> TDKNQTTQNNSSSPLTQVNTTVSVQIGTKALLCCFSIPLTKAVLITWIIKLRGLPSCTIAYKVDTKTNETSCLGRNITWASTPDHSPELQISAVTLQHEGTYTCETVTPE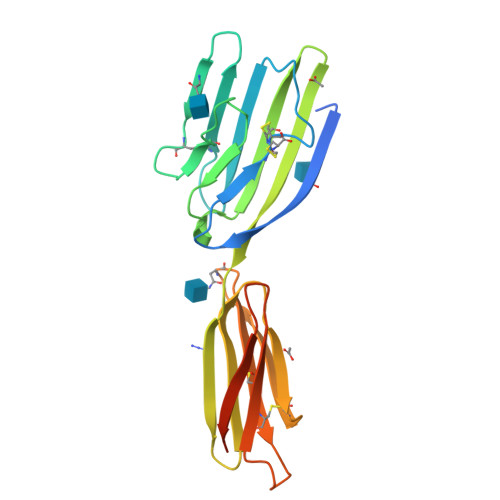GNFEKNYDLQVLVPPEVTYFPEKNRSAVCEAMAGKPAAQISWSPDGDCVTTSESHSNGTVTVRSTCHWEQNNVSDVSCIVSHLTGNQSLSIELGRGGSTRHHHHHH>[14x]GSNLIPTVIETTNRGERAYDIYSRLLKDRIIMLGSQIDDNVANSIV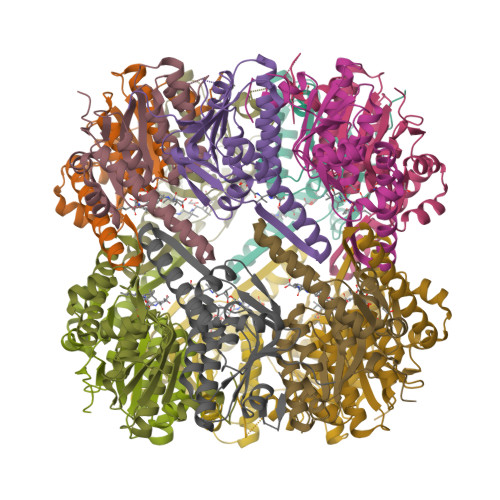SQLLFLQAQDSEKDIYLYINSPGGSVTAGFAIYDTIQHIKPDVQTICIGMAASMGSFLLAAGAKGKRFALPNAEVMIHQPLGGAQGQATEIEIAANHILKTREKLNRILSERTGQSIEKIQKDTDRDNFLTAEEAKEYGLIDEVMVPETK> GPLGSIFPKQYPIINFTTAGATVQSY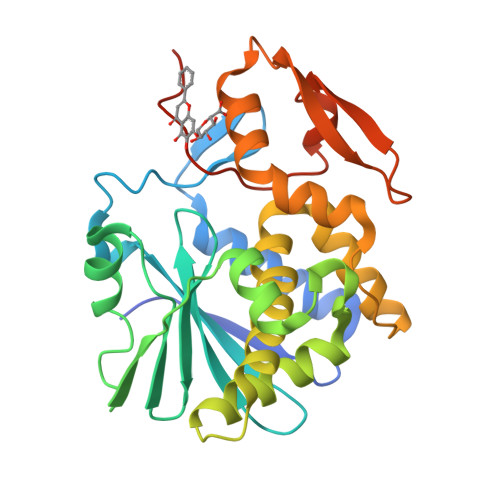TNFIRAVRGRLTTGADVRHEIPVLPNRVGLPINQRFILVELSNHAELSVTLALDVTNAYVVGYRAGNSAYFFHPDNQEDAEAITHLFTDVQNRYTFAFGGNYDRLEQLAGNLRENIELGNGPLEEAISALYYYSTGGTQLPTLARSFIICIQMISEAARFQYIEGEMRTRIRYNRRSAPDPSVITLENSWGRLSTAIQESNQGAFASPIQLQRRNGSKFSVYDVSILIPIIALMVYRCAPPPSSQFLERPHRD Ribonucleotide reductase (RNR) is a key enzyme in all domains of life, utilizing radical chemistry for the synthesis of deoxyribonucleotides by substitution of the 2′ OH-group of a ribose 5′phosphate with a hydrogen. The strictly aerobic class I RNRs are comprised of two homodimeric subunits: a large catalytic subunit R1, where ribonucleotide reduction takes place, and a small radical-generating subunit R2. R2a proteins utilize an oxygen-activated di-ferrous metal site to generate a stable FeIII/FeIII-tyrosyl radical (Y·) cofactor, whereas R2b proteins generate a MnIII/MnIII-Y·. R2c proteins generate a MnIV/FeIII cofactor and the recently discovered class R2d—a MnIV/MnIII cofactor. These dimetal centers reside in a ferritin-like scaffold, and are coordinated by two histidine residues and four carboxylate ligands.

Here we show that the class Ib ribonucleotide reductase R2 protein from Bacillus anthracis spontaneously assembles a Mn/Mn cofactor in vitro, under both aerobic and anoxic conditions, when the metal-free protein is subjected to incubation with MnII and FeII in equal concentrations. To study metal selectivity and cofactor assembly from a mixed MnII and FeII pool in the presence and absence of O2, in the present study we describe apoprotein crystal soaking experiments, subjecting apo BaR2b to a large excess of both MnII and FeII in aerobic and reducing anoxic conditions (in presence of 30 mM sodium dithionite). Site-specific metal quantification by X-ray anomalous dispersion on WT BaR2b revealed that the two sites of the metal center predominantly bind Mn irrespective of the presence or absence of O2 in the experimental setup. Unlike R2lox and R2c, wild-type BaR2b is able to select Mn over Fe in both binding sites. The capability to exclude Fe appears central for a protein requiring a di-Mn cofactor for function. If Mn binds in both positions, neither the wild-type nor the L61G reacts with O2.

>MRAVNWNKKEDDFSLMFWKQNIAQFWTEEEIAVSSDKNTWVQLSKEEQIAYKRVLGGLTLLDTKQGGEGMPLVLVHLENLQAKSVLAFMGAMEEVHAKSYSHIFTTLATEEEIDEIFDWVDTHPLLEKKAGIITSYYRRLLKPEVTKKELYMAMVASVFLESYLFYSGFFYPLYLAGQGKLTASGEIINLIIRDESIHGVFVGILAQQIFAELSAEDQQEVQKETQELLMELYEIEMAYTEEIYTSIGLVEDVNRFVRYNANKGLMNLGLEPKFEEEEINPIVLNGLRTDTKNHDFFSVKGNGYVKATNVEKLSDDDFVFNF[2x]> GPQMDLTSSHTVM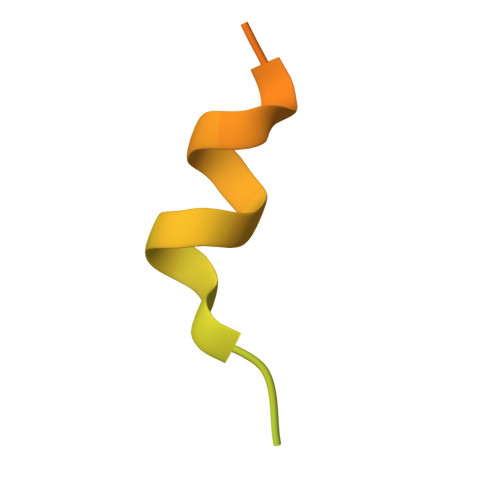ITKGLLDNPISEKSTKIDTTSFLANLKLHTEDSRMKKEVN> GPAMFEARLVQGSILKKVLEALKDLINEACWDISSSGVNLQSMDSSHVSLVQLTLRSEGFDTYRCDRNLAMGVNLTSMSKILKCAGNEDIITLRAEDNADTLALVFEAPNQEKVSDYEMKLMDLDVEQLGIPEQEYSCVVKMPSGEFARICRDLSHIGDAVVISCAKD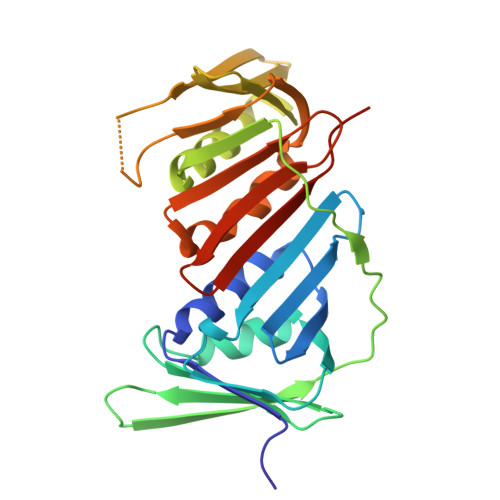GVKFSASGELGNGNIKLSQTSNVDKEEEAVTIEMNEPVQLTFALRYLNFFTKATPLSSTVTLSMSADVPLVVEYKIADMGHLKYYLAPKIEDEEGS>GGDGGEPSQLPHCPSVSPSAQPWTHPGQSQLFADLSREELTAVMRFLTQRLGPGLVDAAQARPSDNCVFSVELQLPPKAAALAHLDRGSPPPAREALAIVFFGRQPQPNVSELVVGPLPHPSYMRDVTVERHGGPLPYHRRPVLFQEYLDIDQMIFNRELPQASGLLHHCCFYKHRGRNLVTMTTAPRGLQSGDRATWFGLYYNISGAGFFLHHVGLELLVNHKALDPARWTIQKVFYQGRYYDSLAQLEAQFEAGLVNVVLIPDNGTGGSWSLKSPVPPGPAPPLQFYPQGPRFSVQGSRVASSLWTFSFGLGAFSGPRIFDVRFQGERLVYEISLQEALAIYGGNSPAAMTTRYVDGGFGMGKYTTPLTRGVDCPYLATYVDW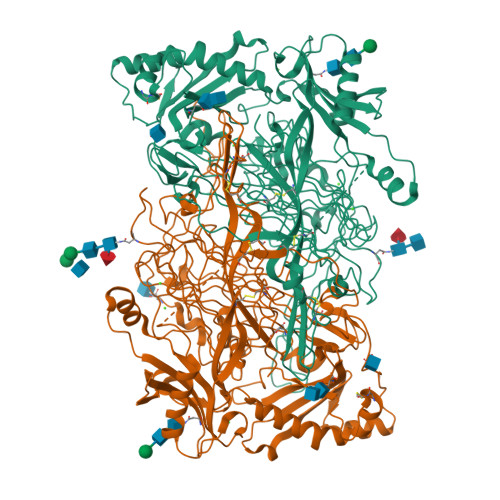HFLLESQAPKTIRDAFCVFEQNQGLPLRRHHSDLYSHYFGGLAETVLVVRSMSTLLNYDYVWDTVFHPSGAIEIRFYATGYISSAFLFGATGKYGNQVSEHTLGTVHTHSAHFKVDLDVAGLENWVWAEDMVFVPMAVPWSPEHQLQRLQVTRKLLEMEEQAAFLVGSATPRYLYLASNHSNKWGHPRGYRIQMLSFAGEPLPQNSSMARGFSWERYQLAVTQRKEEEPSSSSVFNQNDPWAPTVDFSDFINNETIAGKDLVAWVTAGFLHIPHAEDIPNTVTVGNGVGFFLRPYNFFDEDPSFYSADSIYFRGDQDAGACEVNPLACLPQAAACAPDLPAFSHGGFSHN[4x]>[2x]MAEMVETVCGPVPVEQLGKTLIHEHFLFGYPGFQGDVTRGTFREDESLRVAVEAAEKMKRHGIQTVVDPTPNDCGRNPAFLRRVAEETGLNIICATGYYYEGEGAPPYFQFRRLLGTAED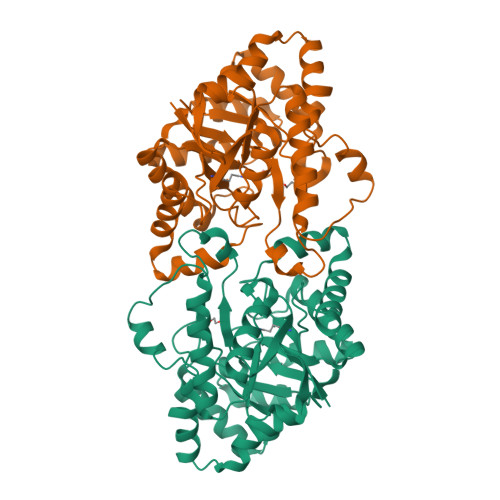DIYDMFMAELTEGIADTGIKAGVIKLASSKGRITEYEKMFFRAAARAQKETGAVIITHTQEGTMGPEQAAYLLEHGADPKKIVIGHMCGNTDPDYHRKTLAYGVYIAFDRFGIQGMVGAPTDEERVRTLLALLRDGYEKQIMLSHDTVNVWLGRPFTLPEPFAEMMKNWHVEHLFVNIIPALKNEGIRDEVLEQMFIGNPAALFSA2-[4-({2-[(2S,5R)-2-(AMINOMETHYL)-5-ETHYNYLPYRROLIDIN-1-YL]-2-OXOETHYL}AMINO)-4-METHYLPIPERIDIN-1-YL]ISONICOTINIC ACID | C21 H29 N5 O3 | 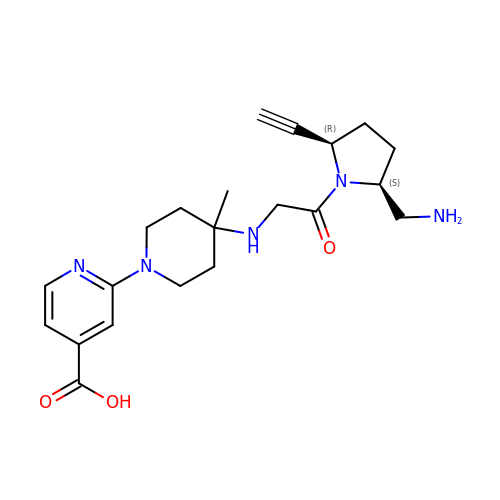SDLYKSXRUIHFDH-IRXDYDNUSA-N> MEGISIYTSDNYTEEMGSGDYDSMKEPCFREENANFNKIFLPTIYSIIFLTGIVGNGLVILVMGYQKKLRSMTDKYRLHLSVADLLFVITLPFWAVDAVANWYFGNFLCKAVHVIYTVNLYSSVLILAFISLDRYLAIVHATNSQRPRKLLAEKVVYVGVWIPALLLTIPDFIFANVSEADDRYICDRFYPNDLWVVVFQFQHIMVGLILPGIVILSCYCIIISKLSHSKGHQKRKALKTTVILILAFFACWLPYYIGISIDSFILLEIIKQGCEFENTVHKWISITEALAFFHCCLNPILYAFLGAKFKTSAQHALTSVSRGSSLKILSKGKRGGHSSVSTESESSSFHSSDY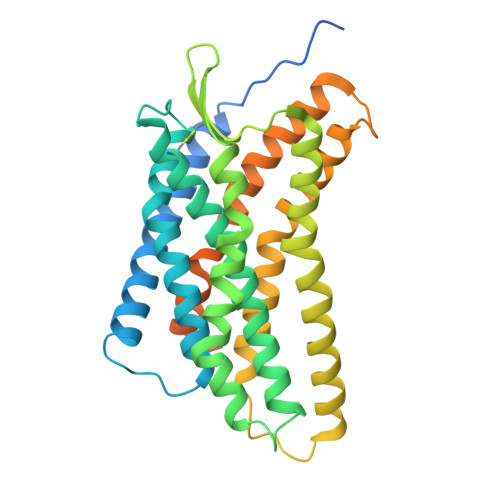KDDDDK N1-CARBOXYPIPERAZINE | C5 H10 N2 O2 | 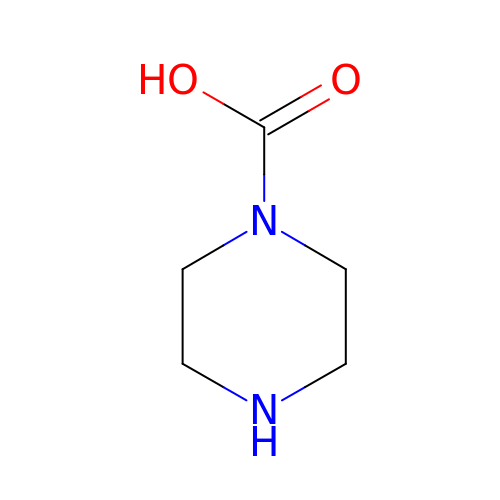RFIOZSIHFNEKFF-UHFFFAOYSA-N>MGSSHHHHHHSQDPNSSSMAERFDNLVEGLTEERAMAVILADPDSLERPVDKYMAATRLGASNSEESLDVLIQAAELDPEHLFNRITRRKAIDALGRRKSPKALPSLFKALKCSDEAAVINSVEAITKIDAPLTEADHEKLLEALKGEDIQKRAVIQAFCRLGVPGVINSISPLQDDSNPLVAGAARAYMSKVALQPDGLEVLIPQLVDPIAGRRRSAVIDLGDAGDVTRLEALVTAPVSMSLRARSAFQLVDPDKTCQVPEKYAELITQLLQDNPQQLKLRKEWICDIEPTEIENNLQHRDEARQYGGASSLMAMPKAERMILINEIKEKLWSDYVTHYYLTAVVGLQGLEERSDLIRLALAETIPQYTKSRIAAAWGCLRLGLVDQKPLLE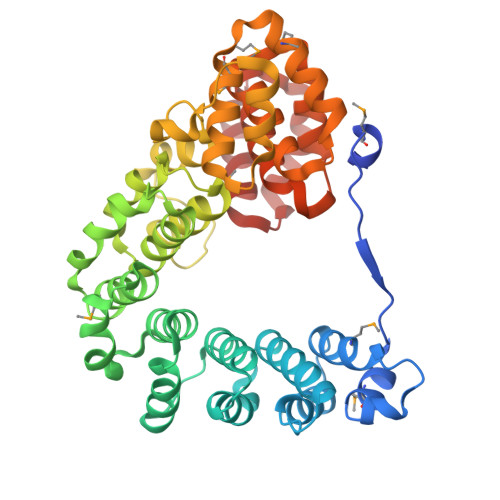ELSVSAFWLPLKWTCQRVLKQLS[2x]>[4x]EDPPACGSIVPRREWRALASECRERLTRPVRYVVVSHTAGSHCDTPASCAQQAQNVQSYHVRNLGWCDVGYNFLIGEDGLVYEGRGWNIKGAHAGPTWNPISIGISFMGNYMNRVPPPRALRAAQNLLACGVALGALRSNYEVKGHRDVQPTLSPGDRLYEIIQTWSHYRA

The 19 kDa peptidoglycan recognition protein (PGRP-S) is one of the four mammalian PGRPs which were originally classified according to their molecular weights as PGRP-S (M.W., 20–25 kDa), PGRP-Iα and PGRP-Iβ (M.W., 40–45 kDa) and PGRP-L (M.W. up to 90 kDa). The significant concentration of PGRP-S has so far been reported in the mammary secretions of camel (Camelus dromedarius) only. As part of the innate immune system, mammary PGRP-S contributes to the protection of animal udder as well as to the new borns against the invading microbes. It recognizes various pathogen-associated molecular patterns (PAMPs) with high affinity.

The A–B and C–D interfaces involve two opposite faces of a monomer leading to the formation of the linear chain with alternating A–B and C–D contacts. The previous studies have shown that LPS, LTA and PGN bind to CPGRP-S at Site-1 which is situated at the C–D contact while mycolic acid and other fatty acids were held at Site-2 at the A–B contact. Having obtained these results, it was pertinent to determine whether CPGRP-S could bind to the components of multiple bacterial cell wall molecules simultaneously through its two independent binding sites or it would bind to only one kind of PAMPs at a time. Therefore, the binding studies of CPGRP-S with LPS and SA were carried out in the presence of each other which showed that LPS and SA bound to CPGRP-S with similar affinities as those reported in the bimolecular interactions. In order to reveal the mode of binding of two different types of cell wall molecules simultaneously, a ternary complex of CPGRP-S with LPS and SA was crystallized. The structure determination of the complex showed that LPS and SA were observed bound to Site-1 and Site-2 respectively. This indicated the binding potential of CPGRP-S to interact with two independent PAMPs through its two separate binding sites, S-1 and S-2.>LEEKKVCQGTSNKLTQLGTFEDHFLSLQRMFNNCEVVLGNLEITYVQRNYDLSFLKTIQEVAGYVLIALNTVERIPLENLQIIRGNMYYENSYALAVLSNYDANKTGLKELPMRNLQEILHGAVRFSNNPALCNVESIQWRDIVSSDFLSNMSMDFQNHLGSCQKCDPSCPNGSCWGAGEENCQKLTKIICAQQCSGRCRGKSPSDCCHNQCAAGCTGPRESDCLVCRKFRDEATCKDTCPPLMLYNPTTYQMDVNPEGKYSFGATCVKKCPRNYVVTDHGSCVRACGAD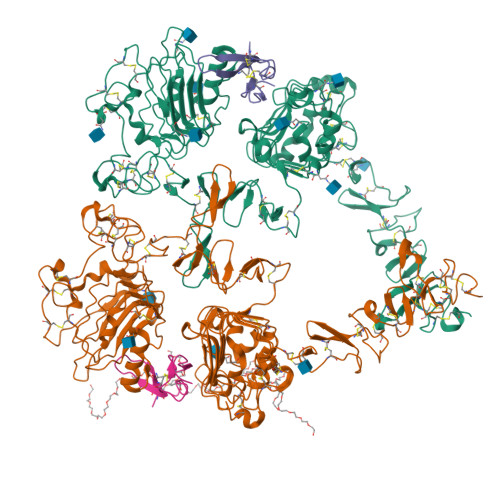SYEMEEDGVRKCKKCEGPCRKVCNGIGIGEFKDSLSINATNIKHFKNCTSISGDLHILPVAFRGDSFTHTPPLDPQELDILKTVKEITGFLLIQAWPENRTDLHAFENLEIIRGRTKQHGQFSLAVVSLNITSLGLRSLKEISDGDVIISGNKNLCYANTINWKKLFGTSGQKTKIISNRGENSCKATGQVCHALCSPEGCWGPEPRDCVSCRNVSRGRECVDKCKLLEGEPREFVENSECIQCHPECLPQAMNITCTGRGPDNCIQCAHYIDGPHCVKTCPAGVMGENNTLVWKYADAGHVCHLCHPNCTYGCTGPGLEGCPT[2x];>ECPLSHDGYCLHDGVCMYIEALDKYACNCVVGYIGERCQYRDLKWWE[2x]> SIYVLSMNRMICDCVSRITGDRVKNIVLIDGAIDPHSYEMVKGDEDRMAMSQLIFCNGLGLEHSASLRKHLEGNPKVVDLGQRLLNKNCFDLLSEEGFPDPHIWTDMRVWGAAVKEMAAALIQQFPQYEEDFQKNADQILSEMEELDRWAARSLSTIPEKNRYLVTGHNAFSYFTRRYLSSDAERVSGEWRSRCISPEGLSPEAQISIRDIMRVVEYISANDVEVVFLEDTLNQDALRKIVSCSKSGQKIRLAKSPLYSDNVCD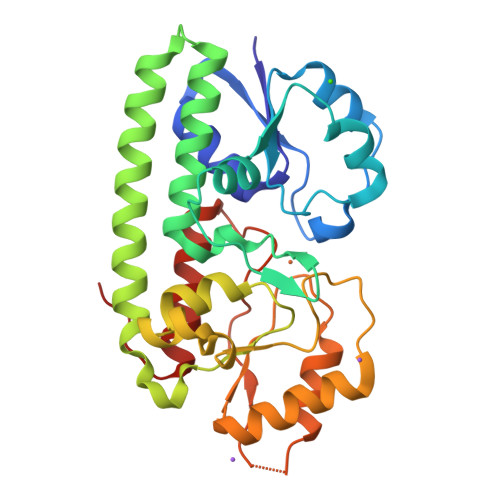NYFSTFQHNVRTITEELGGTVLE>[2x]MGSSLDDEHILSALLQSDDELVGEDSDSEISDHVSEDDVQSDTEEAFIDEVHEVQPTSSGSEILDEQNVIEQPGSSLASNKILTLPQRTIRGKNKHCWSTSKSTRRSRVSALNIVRSQRGPTRMCRNIYDPLLCFKLFFTDEIISEIVKWTNAEISLKRRESMTGATFRDTNEDEIYAFFGILVMTAVRKDNHM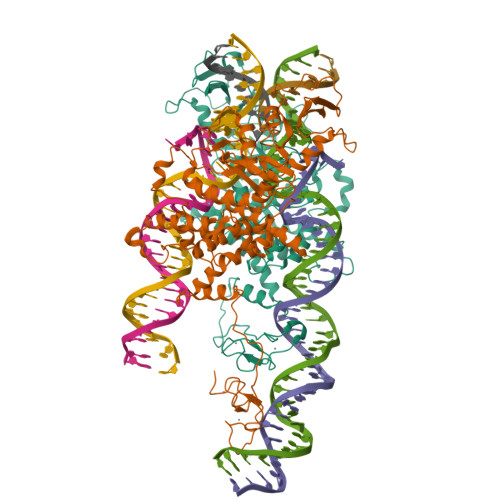STDDLFDRSLSMVYVSVMSRDRFDFLIRCLRMDDKSIRPTLRENDVFTPVRKIWDLFIHQCIQNYTPGAHLTIDEQLLGFRGRCPFRMYIPNKPSKYGIKILMMCDSGTKYMINGMPYLGRGTQTNGVPLGEYYVKELSKPVRGSCRNITCDNWFTSIPLAKNLLQEPYKLTIVGTVRSNKREIPEVLKNSRSRPVGTSMFCFDGPLTLVSYKPKPAKMVYLLSSCDEDASINESTGKPQMVMYYNQTKGGVDTLDQMCSVMTCSRKTNRWPMALLYGMINIACINSFIIYSHNVSSKGEKVQSRKKFMRNLYMSLTSSFMRKRLEAPTLKRYLRDNISNILPNEVPGTSDDSTEEPVTKKRTYCTYCPSKIRRKANASCKKCKKVICREHNIDMCQSCF> GAMAHGIPSQGKVTITVDEYSSNPTQAFTHYNINQSRFQPPHVHMVDPIPYDTPKPAGHTRFVCISDTHSRTDGIQMPYGDILLHTGDFTELGLPSEVKKFNDWLGNLPYEYKIVIAGNHELTFDKEFMADLVKQDYYRFPSVSKLKPEDFDNVQSLLTNSIYLQDSEVTVKGFRIYGAPWTPWFNGWGFNLPRGQSLLDKWNLIPEGTDILMTHGPPLGFRDWVPKE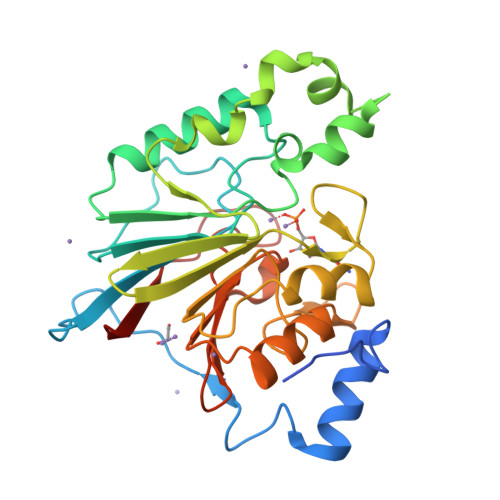LQRVGCVELLNTVQRRVRPKLHVFGHIHEGYGTMTDGYTTYINASTCTVSFQPTNPPIIFDLPNPQGS3-[(4-amino-2-methylpyrimidin-5-yl)methyl]-2-{(1S)-1-hydroxy-1-[(R)-hydroxy(oxo)-lambda~5~-phosphanyl]ethyl}-5-(2-{[(S)-hydroxy(phosphonooxy)phosphoryl]oxy}ethyl)-4-methyl-1,3-thiazol-3-ium 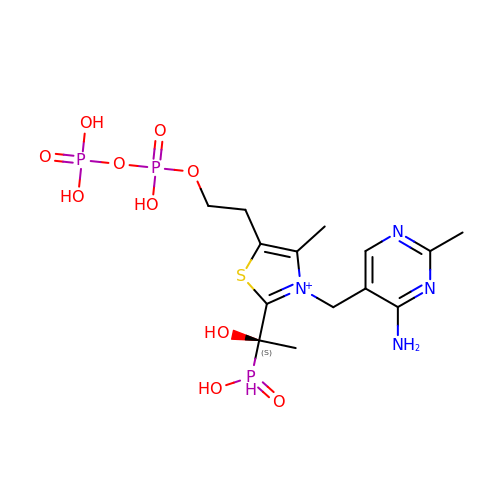| C14 H24 N4 O10 P3 S | CAOFPOCACDCAFN-AWEZNQCLSA-O> MVITKIVGHID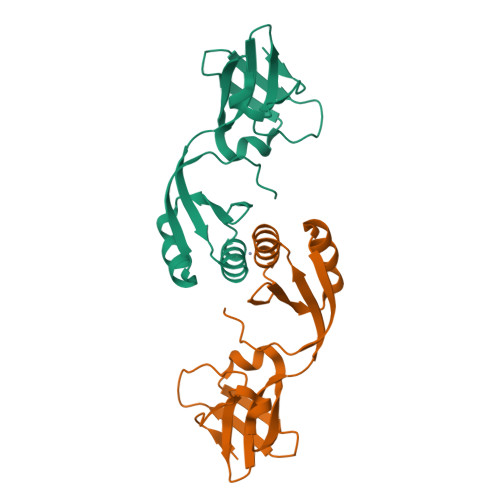DLSHQIKKVDWLEVEWEDLNKRILRKETENGTDIAIKLENSGTLRYGDVLYESDDTLIAIRTKLEKVYVIKPQTMQEMGKMAFEIGNRHTMCIIEDDEILVRYDKTLEKLIDEVGVSYEQSERRFKEPFKYRGHQH>[2x]MMQQSRPASDPQVVEAARKEGRLIIYSATDQSSAQALLDDFRKLYPFIQIEYNDLGTQAIYDRFVSETAAGASSADLLWSSAMELQVKLASEGYALPYDSPEAKNWPANARLGNLAYSTTLEPAVVVYNKRFLKPEEVP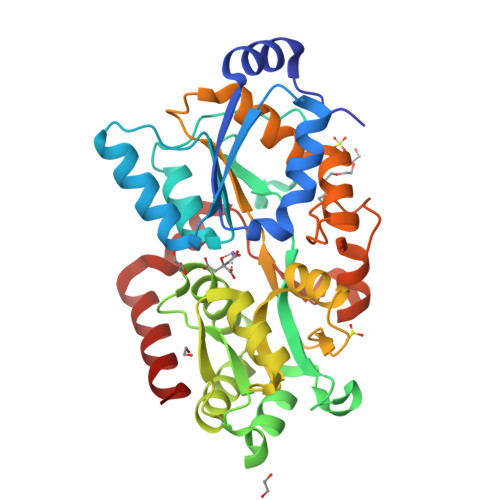TTREGLARLLQEPRMRGRVATWDPERSAVGFTILKADYDRFPAFQELARAFGKAQAALYSSTGAAFEKVISGEHYLAYGFFGSYALLRQRTVKDLGIAYLTDGTVAIQRVAFINKRAAHPNAAKLFLDYLLSLRGQNLMAYTALIFARRETVVGEATPQALYKAVGGKDKVYAIPVSTEILKNLDPAERMRFLTFWRQAVRGQ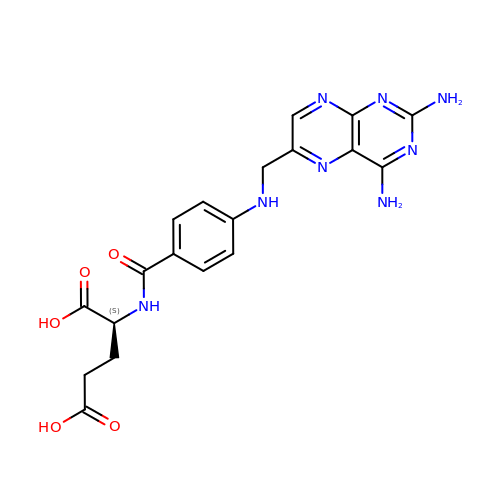Aminopterin | C19 H20 N8 O5 | TVZGACDUOSZQKY-LBPRGKRZSA-N>MHHHHHHSSGLVPRGSLRVGNRYRLGRKIGSGSFGDIYLGTDIAAGEEVAIKLECVKTKHPQLHIESKIYKMMQGGVGIPTIRWCGAEGDYNVMVMELLGPSLEDLFNFCSRKFSLKTVLLLADQMISRIEYIHSKNFIHRDVKPDNFLMGLGKKGNLVYIIDFGLAKKYRDARTHQHIPYRENKNLTGTARYASINTHLGIEQSRRDDLESLGYVLMYFNLGSLPWQGLKAATKRQK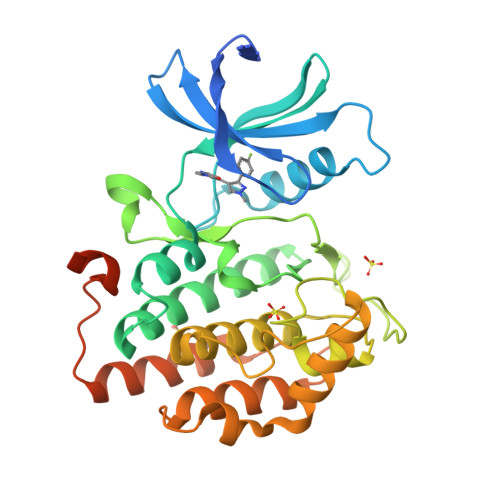YERISEKKMSTPIEVLCKGYPSEFATYLNFCRSLRFDDKPDYSYLRQLFRNLFHRQGFSYDYVFDWNMLKFGASRAADDAERERRDREERLRH[4x]>FKTIKSDEIFAAAQKLMPGGVSSPVRAFKSVGGQPIVFDRVKDAYAWDVDGNRYIDYVGTWGPAICGHAHPEVIEALKVAMEKGTSFGAPCALENVLAEMVNDAVPSIEMVRFVNSGTEACMAVLRIMRAYTGRDKIIKFEGCYHGHADMFLVKAGSGVATLGLPSSPGVPKKTTANTLTTPYNDLEAVKALFAENPGEIAGVILEPIVGNSGFIVPDAGFLEGLREITLEHDALLVFDEVITGFRIAYGGVQEKFGVTPDLTTLGKIIGGGLPVGAYGGKREIMQL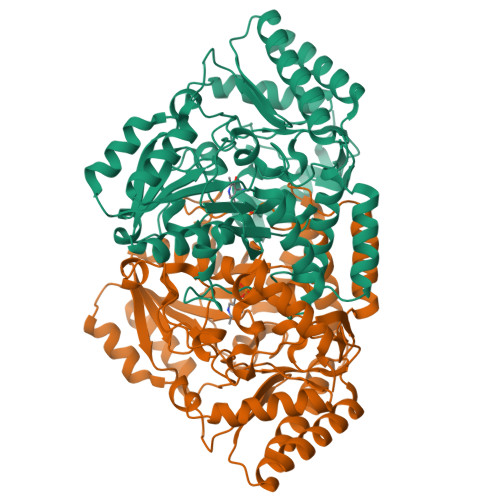VAPAGPMYQAGTLSGNPLAMTAGIKTLELLRQPGTYEYLDQITKRLSDGLLAIAQETGHAACGGQVSGMFGFFFTEGPVHNYEDAKKSDLQKFSRFHRGMLEQGIYLAPSQFEAGFTSLAHTEEDIDATLAAARTVMSAL[2x]> GSHMMGNKQTVFTHEQLEAYQDCTFFTRKEIM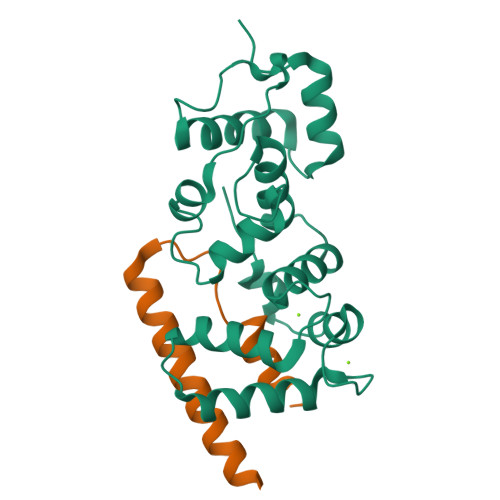RLFYRYQDLAPQLVPLDYTTCPDVKVPYELIGSMPELKDNPFRQRIAQVFSEDGDGHMTLDNFLDMFSVMSEMAPRDLKAYYAFKIYDFNNDDYICAWDLEQTVTKLTRGELSAEEVSLVCEKVLDEADGDHDGRLSLEDFQNMILRAPDFLSTFHIRI;> GGGDDNTFNFSWKVFCSWDYLIGNPETADNKFNSITMNFKEAIIEERAAQVEENI>MKETWWETWWTEWSQPKKKRKVMSSATSFFDFKVPDGADNEVDLSQYKGKVVLVVNTASKCGFTYQYKNLESVYQAIKKEYPDDFVVLGFPCNQFGSQEPGSNEEIQNFCSLEQKVTFPVMGKINVNGDDAHPLYKWLKKEKPGLLGLERVKW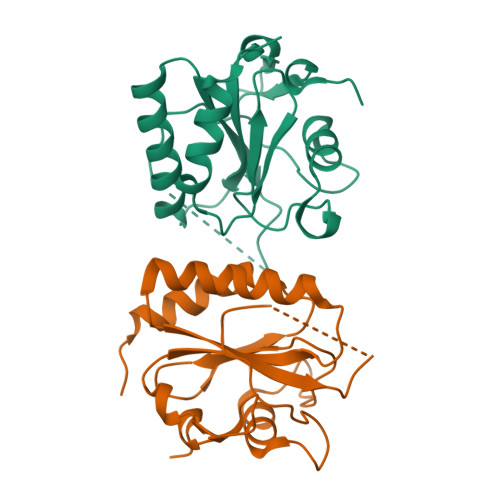NFEKFLIGRDGKVIGRWASTTEPEKIQDKIIEAIKQPAP[2x]>GAGAGALSGNSPHELKNAAQRAADWLVERQRPNGALPSRTAVIESCYKGMWALHTAGHTQAASAVADYVTSLLQPDGDIPQPREERYFLDVHYLYANGYLTIGAHVLGRFGLSRKLMSFVETMRNPATGGFRSHGPAIPGDGRCDSVSTSISGLAALYTGRVDTARSAADFLGSLWVGQPDRKNVFHAVADASGAVLTSDDAVAVQVRKAEGDWYFIGLPAFFLTALYEATEDRAYLDLATDLMTYMDEDCDEDAFVDSSCGKAGVAAALLYRLTGRPRYREIAEGIGTLLCE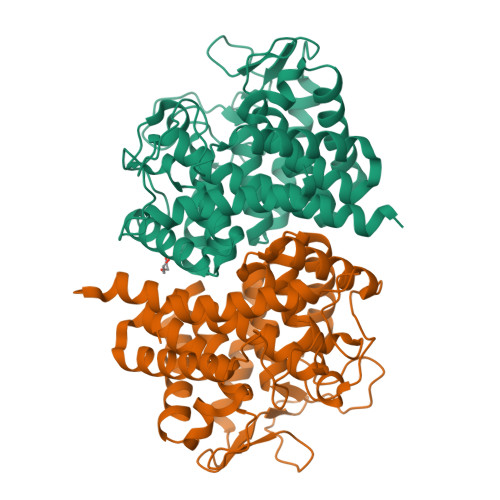RQSPYGYWSEEETGDVADLFWGDLDMTAEYVLWLDLIGRNLASGERVWAGKR[6x]>ANIVGGIEYSINNASLCSVGFSVTRGATKGFVTAGHCGTVNATARIGGAVVGTFAARVFPGNDRAWVSLTSAQTLLPRVANGSSFVTVRGSTEAAVGAAVCRSGRTTGYQCGTITAKNVTANYAEGAVRGLTQGNACMGRGDSGGSWITSAGQAQGVASGGNVQSNGNNCGIPASQRSSLFERLQPILSQYGLSLVTG[2x];>[2x]ADQVDPQLKFAMQRDLGIFPTQLPQYLQTEKLARTQAAAIEREFGAQFAGSWIERNEDGSFKLVAATSGARKSSTLGGVEVRNVRYSLKQLQSAMEQLDAGANARVKGVSKP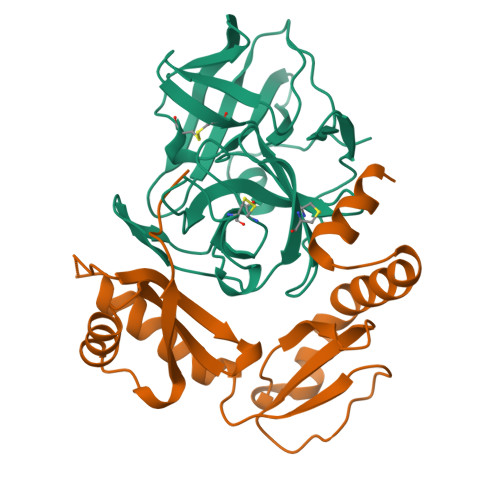LDGVQSWYVDPRSNAVVVKVDDGATDAGVDFVALSGADSAQVRIESSPGKLQTT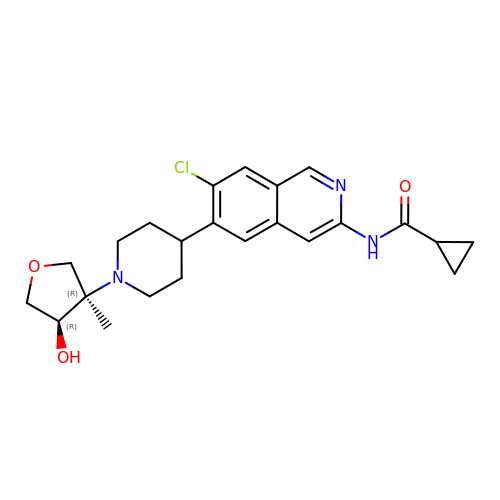N-(7-chloro-6-{1-[(3R,4R)-4-hydroxy-3-methyloxolan-3-yl]piperidin-4-yl}isoquinolin-3-yl)cyclopropanecarboxamide | C23 H28 Cl N3 O3 | AUWBKRNKWPJDOB-NZQKXSOJSA-N>[8x]SNAARGHRHTCKVMVLKEEAAGSERALALDMREGQRVFHSLIVHFENDIPVQIEDRFVNAQVAPDYLKQDFTLQTP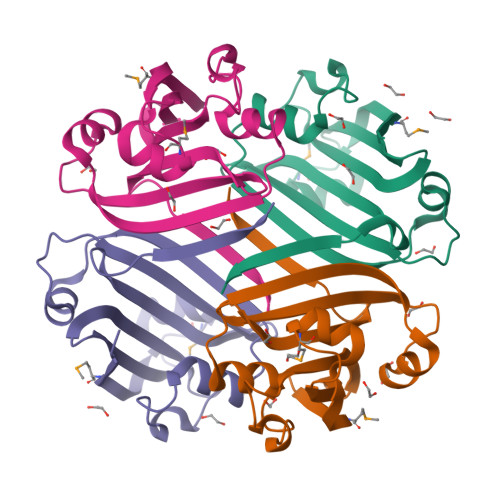YAYLSQVAPLTEGEHVVEAILAEADECKLLQIDAGEPCLLIRRRTWSGRQPVTAARLIHPGSRHRLEGRFTK>MSDEQKKPEQIHRRDILKWGAMAGAAVAIGASGLGGLAPLVQTAAKPSKKDEKEEEQIVPFYGKHQAGITTAHQTYVYFAALDVTAKDKSDIITLFRNWTSLTQMLTSGKKMSAEQRNQYLPPQDTGESADLSPSNLTVTFGFGPGFFEKDGKDRFGLKSKKPKHLAALPAMPNDNLDEKQGGGDICIQVCADDEQVAFHALRNLLNQAVGTCEVRFVNKGFLSGGKNGETPRNLFGFKDGTGNQSTKDDTLMNSIVWIQSGEPDWMTGGTYMAFRKIKMFLEVWDRSSLKDQEDTFGRRKSSGAPFGQKKETDPVKLNQIPSNSHVSLAKSTGKQILRRAFSYTEGLDPKTGYMDAGLLFISFQKNPDNQFIPMLKALSAKDALNEYTQTIGSALYACPGGCKKGEYIAQRLLES[2x]

Bacillus subtilis BsDyP belongs to class I of the dye-decolorizing peroxidase (DyP) family of enzymes and is an interesting biocatalyst due to its high redox potential, broad substrate spectrum and thermostability. DyPs are a family of microbial heme peroxidases that display structural features analogous to chlorite dismutases with an α + β ferredoxin-like fold. In BsDyP, the heme cofactor is partially buried in a predominantly hydrophobic pocket lined by the conserved proximal ligand H326 and catalytic distal residues D240 and R339. Access to the heme from the surface, as defined using a 1.4-Å rolling probe, is made through a distal tunnel and an open wide cavity.

We deleted the N-terminal sequence of BsDyP to achieve homogeneous preparations of recombinant enzyme. The truncated enzyme shows spectroscopic and kinetic properties comparable to those of an intact enzyme. This form (named hereafter wild-type BsDyP) was used throughout this work. To investigate the structural consequences of evolving the wild type to 5G5, the X-ray crystal structures of 5G5 and the wild type were solved at 2.10 and 2.49 Å resolution, respectively. The wild type crystallized in the trigonal P3121 space group with two molecules per asymmetric unit. These two subunits have an r.m.s.d. of 0.31 Å between Cα atoms. K317 (and D314 from loop 2) establishes salt bridges with D250 (and K248) from symmetry-related molecules in the wild-type crystal structure. The catalytic D240 and R339 residues are part of the tunnel, and three water molecules were found in this pathway in the wild-type structure (and four in the 5G5 structure). The wild-type BsDyP displays a GdnHCl mid-point concentration (where 50% of molecules are unfolded) of 1.4 M, and the native state is more stable than the unfolded state by 7 kcal mol−1. Furthermore, the kinetic stability, which quantifies the amount of enzyme that loses activity irreversibly during incubation at a certain temperature, owing to misfolding, protein aggregation and covalent changes, reveals that the wild-type enzyme is clearly more stable than the variants with a 4-fold higher half-life at 40 °C.>GPLGSEEDVPENNGILISIKEVINAEFSRDGTIHSSELKGVLELRINDHDLSHSNLKLADSIDVRDKSFQFKTHPNIDKQSFLSTKLISLRDKSKAFPANDQSLGVLRWRKVAPAEDDSLIPLTLTTAVSPSESQQGFDVIIEYESVLETELADVIFTIPVFPQEPVDINTESSTCSDAEVVNMDQEMGTSIKISKIAANDAGALAFTIEAPYEDALYPMTVSFQESTRDKLAKSFTGMAIQSVVMANDHDQELPYDVITSLKSDEYLVQ[4x];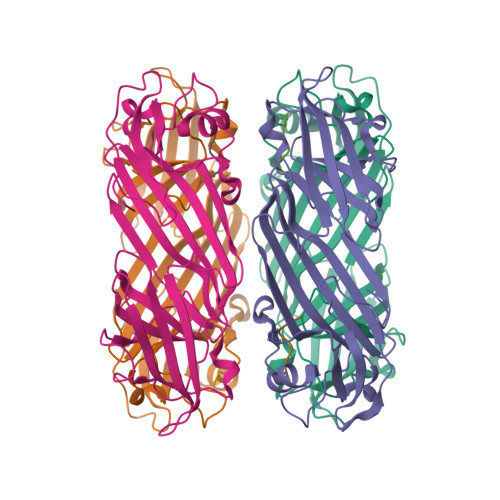>DDWNWEVED[4x]> MSVIKSDMKIKLRMEGTVNGHKFVIEGEGEGKPYEGTQTMNLKVKEGAPLPFAYDILTTVFHYGNRVFAKYPKHIPDYFKQSFPEGYSWERSMTFEDGGICTARNDITLEGDCFFNEIRFDGVNFPPNGPVMQKKTLKWEPSTEKMYVRDGVLTGDINMALLLEGGGHYRCDFKTTYKAKKGVQLPDYHFVDHCIEILSHDKDYNNVKLYEHAVAH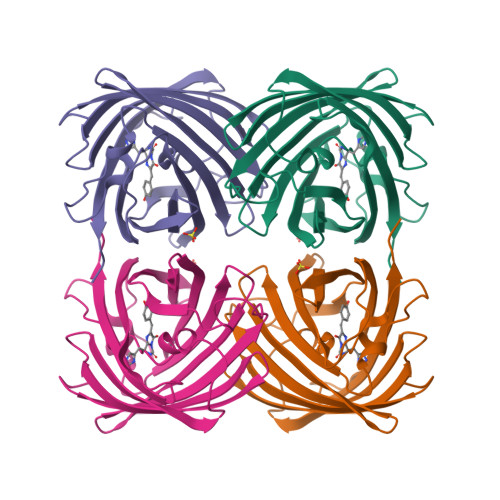SGLPRQAKHHHHHH Among purple photosynthetic bacteria, the transcription factor CrtJ is a major regulator of photosystem gene expression. Recently, CrtJ’s activity was shown to be modulated by two size variants of a B12 binding co-regulator called SAerR and LAerR in Rhodobacter capsulatus. The short form, SAerR, promotes CrtJ repression, while the longer variant, LAerR, converts CrtJ into an activator.

In this study, we solved the crystal structure of R. capsulatus SAerR at a 2.25 Å resolution. The solved crystal structure of SAerR containing bound cobalamin has a four-helix bundle cap followed by an α/β Rossman fold. A flexible loop between the four-helix bundle and the α/β Rossman fold is not resolved in the structure. B12 is nestled between the four-helix bundle cap on the left and the Rossman fold on the right. The corrin ring is anchored in place by His145 in the Rossman fold that functions as the lower ligand to the Co in cobalamin. In SAerR, His10 is not present, as this variant is 40 AA shorter at the amino terminus relative to LAerR. In this case, the best fit for an upper axial ligand in the SAerR electron density map is an atom of Cl (dappled ball in Figure 2B,C). SAerR crystals were grown in a high concentration of NaCl, so Cl appears to have replaced the upper ligand –OH that was originally present in hydroxycobalamin that was light-attached to SAerR. Two additional Cl atoms were found in the structure, as well as a molecule of the additive 1,6- hexandiol that we used for the optimization of crystal growth. Analysis of the region near the upper Cl axial ligand shows that it is protected by two aromatic residues, Trp94 and Phe101, in SAerR.

> SLQTVLVNRMVELATGPELGAMDLLFDEFRAAHVPVEEMATHYIPEAARQIGAAWDSDRIGFAQVTIAISRLQELLHALQTLVTADSVGCANGATVLLIVPPGEQHTLGALIVAMELRRRGVSVRIVFAPGLSDLSRLMATTRFDAALITVGSMDRVEICAKLVKTLSSLTKGRMRVAIGGAIVSQRAEALARTGADLVTNDLSLVISEFSLV>MAEKIKINNNVFIYPMPVTLLGANVKGKANLMALGWVSRVNANPPMLGVGVNKSHYTPEGIAENGSFSVNFPYSGMVKKTDYCGLVSGEKVDKSGLFEVFYGELKTAPMIKECTLNLECRVVETLEFPTNYFFVGEIIAAYSEEQYLIQGKPDIKKMDPLLLTMPDNSYWTVGDYAGAALKTGKSLMEKRHHHHHH[2x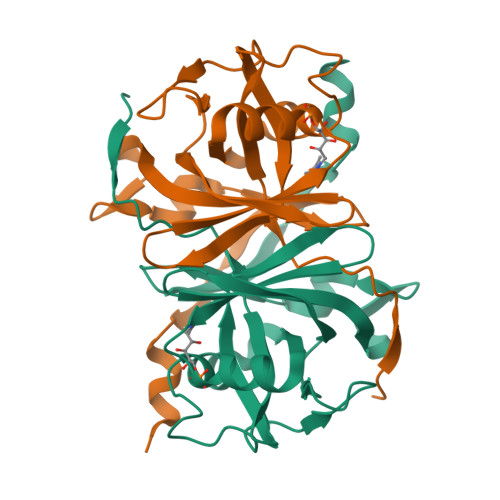]> TPLHSSTLTPMHLRKAKLMFFWVRYPSSAVLKMYFPDIKFNKNNTAQLVKWFSNFREFYYIQMEKYARQAVTEGIKTPDDLLIAGDSELYRVLNLHYNRNNHIEVPQNFRFVVESTLREFFRAIQGGKDT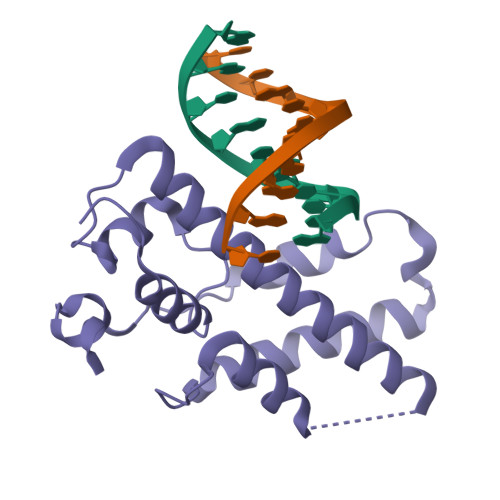EQSWKKSIYKIISRMDDPVPEYFKSPNFLEQLE> MENFTALFGAQADPPPPPTALGFGPGKPPPPPPPPAGGGPGTAPPPTAATAPPGADKSGAGCGPFYLMRELPGSTELTGSTNLITHYNLEQAYNKFCGKKVKEKLSNFLPDLPGMIDLPGSHDNSSLRSLIEKPPILS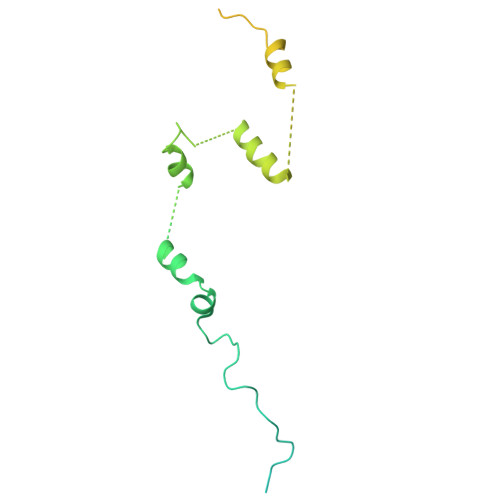SSFNPITGTMLAGFRLHTGPLPEQCRLMHIQPPKKKNKHKHKQSRTQDPVPPETPSDSDHKKKKKKKEEDPDRKRKKKEKKKKKNRHSPDHPGMGSSQASSSSSLR> MFFIKDLSLNITLHPSFFGPRMKQYLKTKLLEEVEGSCTGKFGYILCVLDYDNIDIQRGRILPTDGSA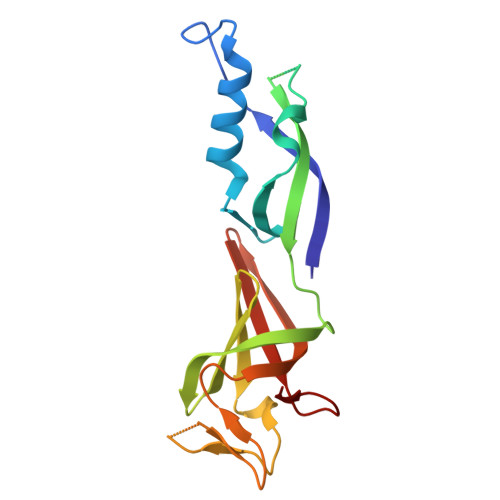EFNVKYRAVVFKPFKGEVVDGTVVSCSQHGFEVQVGPMKVFVTKHLMPQDLTFNAGSNPPSYQSSEDVITIKSRIRVKIEGCISQVSSIHAIGSIKEDYLGAI>GSHHMTGTIETTGNISAEKGGSIILQCHLSSTTAQVTQVNWEQQDQLLAICNADLGWHISPSFKDRVAPGPGLGLTL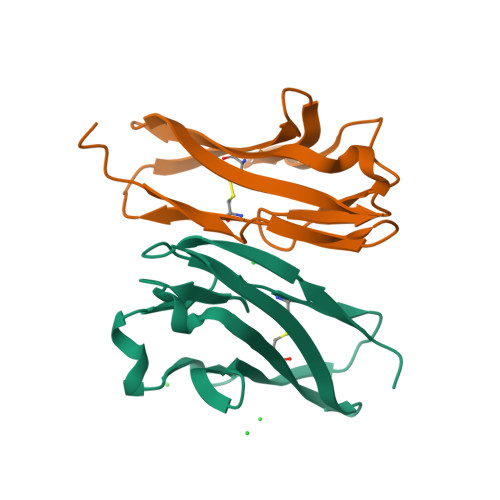QSLTVNDTGEYFCIYHTYPDGTYTGRIFLEVLE[4x]> MKEFRPGDKVVLPPYGVGVVAGIAQRSVSGVSRAYYQVDFPGSRSKAYVPVEAPHSVGLRKALAPEEVPVILDLLKNGRMPLPKQWAARHRKTSEILADGNPYRIAQMAGQLRAWEVERGLPDLDRQALRRAIHLLA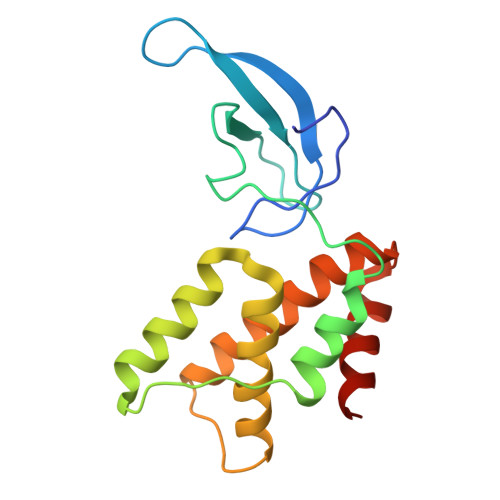EEVAQSLEITVQEAKRLFEEAWGEELN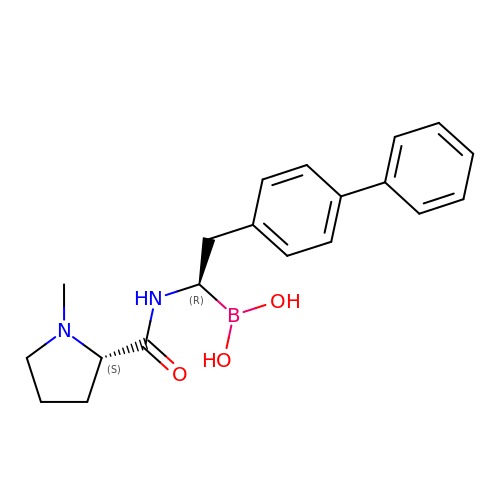N-[(1R)-2-([1,1'-biphenyl]-4-yl)-1-boronoethyl]-1-methyl-L-prolinamide | C20 H25 B N2 O3 | VGGVSZZQWVUBBQ-OALUTQOASA-N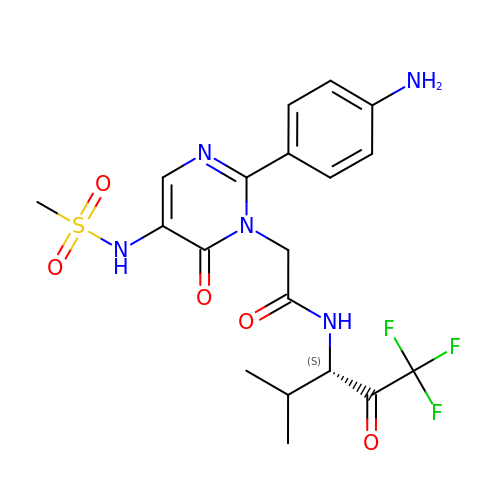2-[5-METHANESULFONYLAMINO-2-(4-AMINOPHENYL)-6-OXO-1,6-DIHYDRO-1-PYRIMIDINYL]-N-(3,3,3-TRIFLUORO-1-ISOPROPYL-2-OXOPROPYL)ACETAMIDE | C19 H22 F3 N5 O5 S | JWSWTHSJMGVOKE-HNNXBMFYSA-N> GNNYVYIDPTQLPYDHKWEFPRNRLSFGKTLGAGAFGKVVEATAYGLIKSDAAMTVAVKMLKPSAHLTEREALMSELKVLSYLGNHMNIVNLLGACTIGGPTLVITEYCCYGDLLNFLRRKRDSFICSKTSPAIMEDDELALDLEDLLSFSYQVAKGMAFLASKNCIHRDLAARNILLTHGRITKICDFGLARDIKNDSNYVVKGNARLPVKWMAPESIFNCVYTFESDVWSYGIFLWELFSL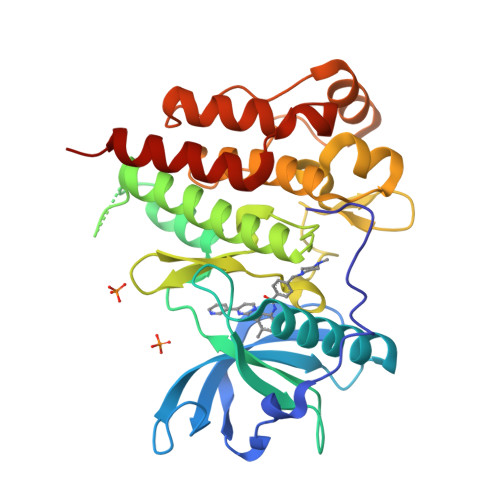GSSPYPGMPVDSKFYKMIKEGFRMLSPEHAPAEMYDIMKTCWDADPLKRPTFKQIVQLIEKQISESTNHI>MAS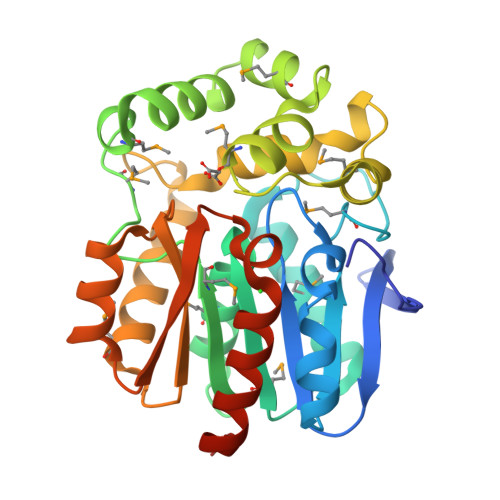SSEFPFAKRTVEVEGATIAYVDEGSGQPVLFLHGNPTSSYLWRNIIPYVVAAGYRAVAPDLIGMGDSAKPDIEYRLQDHVAYMDGFIDALGLDDMVLVIHDWGSVIGMRHARLNPDRVAAVAFMEALVPPALPMPSYEAMGPQLGPLFRDLRTADVGEKMVLDGNFFVETILPEMGVVRSLSEAEMAAYRAPFPTRQSRLPTLQWPREVPIGGEPAFAEAEVLKNGEWLMASPIPKLLFHAEPGALAPKPVVDYLSENVPNLEVRFVGAGTHFLQEDHPHLIGQGIADWLRRNKPHASLEHHHHHH[2x]>[4x]SYSTLANFPVQARNDNISPWTITGFADADSSFMLTVSKDSKRNTGWSVRPRFRIGLHNKDVTILKSIREYLGAGIITSDIDARIRFESLKELEVVINHFDKYPLITQKRADYLLFKKAFYLIKNKEHLTEEGLNQILTLKASLNLGLSEELKEAFPNTI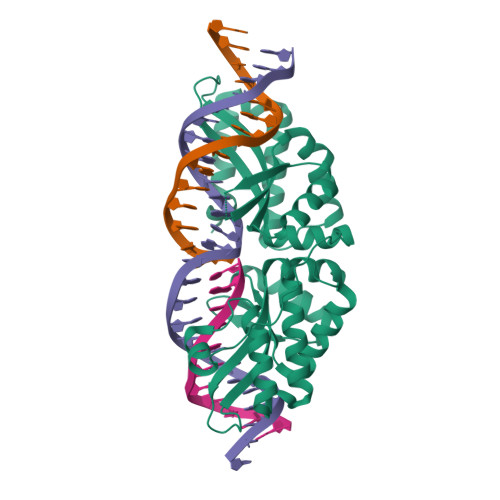PAERLLVTGQEIPDSNWVAGFTAGEGSFYIRIAKNSTLKTGYQVQSVFQITQDTRDIELMKNLISYLNCGNIRIRKYKGSEGIHDTCVDLVVTNLNDIKEKIIPFFNKNHIIGVKLQDYRDWCKVVTLIDNKEHLTSEGLEKIQKIKEGMNRGRSL>[2x]GNLREVRYHDEERPYFIDWDFALRKSGANQTESSMHMQSVVPSSPATPVENDFKRIHSISDMTYLARRTRDEPIRKGVIVPCKDLLDAEEALSRALEVLPLAHKETKDKDRKQQPGIA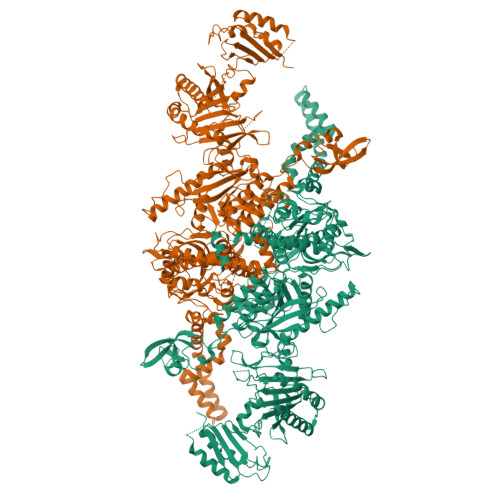ADLAQRRRPGTPLRLEGIGELSAVVNVAVRDAEGKNDEEILALIKPWVQNSKADLLARRVRRLTFICGRNDGSYPSYYTFRGPDYAEDDSIRHIEPSLAFQLELGRLSKFKLTPVFTQNKNIHVYEAVGRGVETDRRYFTRAVVRPGRLRDEISTAEYLISEADRVVNDIFDALEIIGTNKTDLNHMFINFSHTFQVTADEVAESLQGFLDRFGPRGWRLRVHQVEIRINCMRSDNNDENDTMPLRVIITNTSGFVIQIELYEEKLSEKGEWVYYYVSGNAKIGSMHLLPVSTPYPTKNWLQPKRYKAHILGTQYVYDFPELFRQAIQNSWTEAVKKIPSLAAKQPAIGECIDYNELVLGDQDNLAEVSREPGMNSTGMVGWLINARTPEYPDGRKFIVVANDITFKIGSFGPKEDTFFFKCTELARKMGIPRIYLSANSGARLGLAEELMPHFNVAWNDPAKPEAGFKYLYLSDEAKRRFENEVITEEIVEDGEKRHKIITIVGAEEGLGVECLRGSGLIAGATSRAYNDIFTCTLVTCRSVGIGAYLVRLGQRAVQVEGQPIILTGAPALNSLLGREVYTSNLQLGGTQIMYRNGVSHLTAKDDFDGVTKIVQWLSFIPDQRNNPLPILSPSPDPWDRDVVYTPPYKQTYDVRWMIAGKEDEDGFQPGLFDKDSFVETLGGWARTVVVGRARLGGIPMGVIAVETRTIENITPADPANPDSIEQVTNEAGGVWYPNSAFKTAQAINDFNYGEQLPLMILANWRGFSGGQRDMYNEVLKYGSFIVDALTRFEKPIFIYIPPHGELRGGSWVVVDPTINPASMEMYADEEARGGVLEPEGIIPIKYKKDKQLETMARLDPVYRSLKKEMAKEGLSKEESDNIKKKMQQREELLLPIYHQICVQFADLHDRAGRMKAKGVIRQSLQWRQSRRFFYWRVRRRLIEDDILRRIEEAINPAGKRRHDPENTSLAASPETRSPHLVQLESWVGIPGFKTNDREVVEWYEQNQDRINEKLEKLKKESIADQMRELLRXXXXXXXXXXXX>AQKSVKISDDISITQLSDKVYTYVSLAEIEGWGMVPSNGMIVINNHQAALLDTPINDAQTETLVNWVADSLHAKVTTFIPNHWHGDCIGGLGYLQKKGVQSYANQMTIDLAKEKGLPVPEHGFTDSLTVSLDGMPLQCYYLGGGHATDNIVVWLPTENILFGGCMLKDNQATSIGNISDADVTAWPKTLDKVKAKFPSARYVVPGHGDYG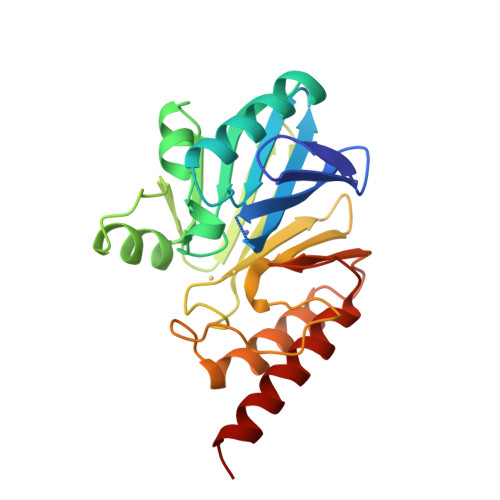GTELIEHTKQIVNQYIESTSKP[2x]> SWRHIRAEGLDSSYTVLFGKAEADEIFQELEKEVEYFTGALARVQVFGKWHSVPRKQATYGDAGLTYTFSGLTLSPKPWIPVLERIRDHVSGVTGQTFNFVLINRYKDGSDHICEHRDDERELAPGSPIASVSFGASRDFVFRHKDSRGKSPSRRVAVVRLPLAHGSLLMMNHPTNTHWYHSLPVRKKVLAPRVNLTFRKIL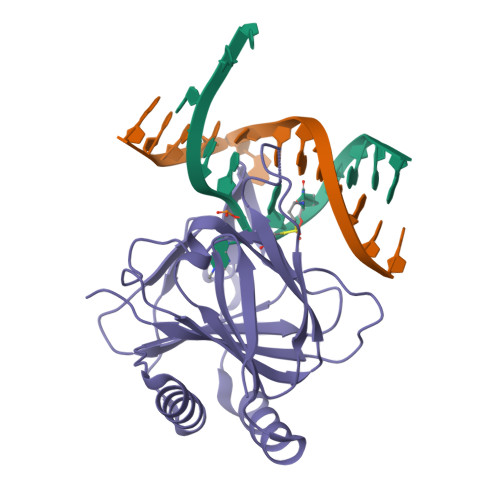L Especially, exposure or modification of N-terminal amino acid residues can mediate protein degradation and the resultant proteolytic procedure is called the N-degron pathway (formerly the N-end rule pathway). Two tertiary degrons, Asn and Gln, are hydrolyzed into the secondary degron Asp and Glu by N-terminal asparagine amidohydrolase 1 (NTAN1) and N-terminal glutamine amidohydrolase 1 (NTAQ1), respectively. In multicellular eukaryotes, Nt-Asn and Nt-Gln are deamidated by NTAN1-encoded NtN-amidase and NTAQ1-encoded NtQ-amidase, respectively. In this study, the crystal structure of NTAN1, the last veiled structure among three amidases in the N-degron pathway, was elucidated.

Although yNta1, NTAQ1, and NTAN1 do appear to share catalytic functions commonly involving a conserved Cys residue critical for the deamidation activity, they exhibit low sequence similarity to each other.

>MPLLVEGRRVRLPQSAGDLVRAHPPLEERARLLRGQSVQQVGPQGLLYVQQRELAVTSPKDGSISILGSDDATTSHIVVLRHTGNGATCLTHCDGTDTKAEVPLIMNSIKSFSDHAQCGRLEVHLVGGFSDDRQLSQKLTHQLLSEFDRQEDDIHLVTLCVTELNDREENENHFPVIYGIAVNIKTAEIYRASFQDRGPEEQLRAARTLAGGPMISIYDAETEQLRIGPYSWTPFPHVDFWLHQDDKQILENLSTSPLAEPPHFVEHIRSTLMFLKKHPSPAHTLFSGNKALLYKKNEDGLWEKISSPGSLEHHHHHH[2x]>[2x]CGCGAT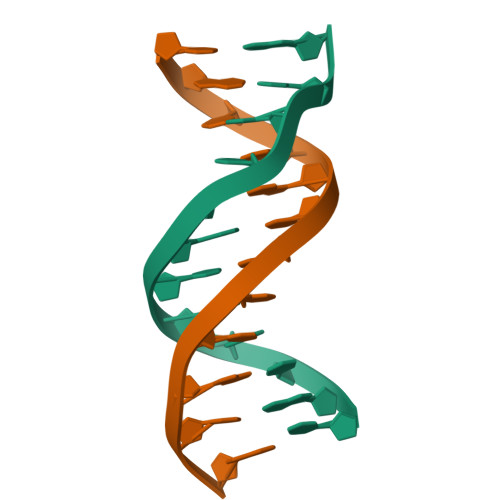ATCGCG>[2x]MKTAALFVSKEFEEEAIALVEGANYKVTSIYKLPKSPNVKFYIQYDKLQQIKNDEEISTLIIFEQLKPRHFINIRRELKGKEVLDKILLLLEIFALHAGSKEAKMQIELARLKYELPIIKETYTKSKIGEQQGPLGAGTYGVESTIKFYKRRINKLMKELESIKIFKEKSIESNKRNNIPSIGIVGYTNSGKTSLFNSLTGLTQKVDTKLFTTMSPKRYAIPINNRKIMLVDTVPF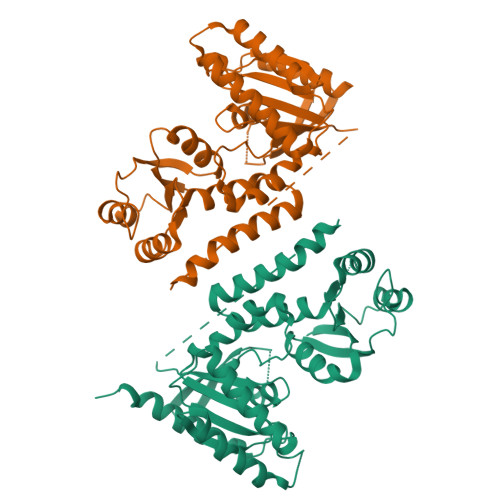IRGIPPQIVDAFFVTLSEAKYSDALILVIDSTFSENLLIETLQSSFEILREIGVSGKPILVTLNKIDKINGDLYKKLDLVEKLSKELYSPIFDVIPISALKRTNLELLRDKIYQLATQLSLEHHHHHH> QDSTSDLIPAPPLSKVPLQQNFQDNQFHGKWYVVGLAGNEVLREDKDPMKMWATIYELEEDKSYNVTIVMPLAEKCEYLFQTFVPGSQPGEFTL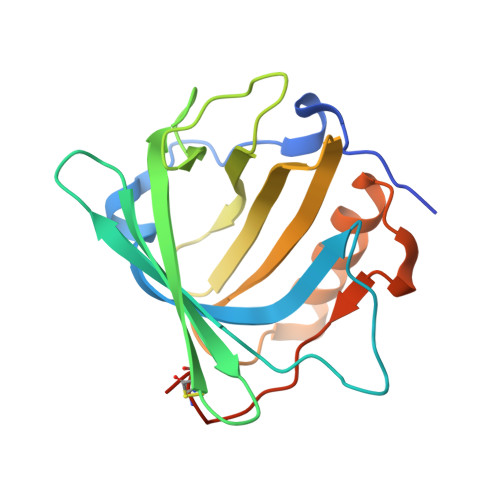GGIKSGPGRTSGLVRVVSTNYNQHAMVFFKVVWQNREVFWVTLYGRTKELTSELKENFIRFSKSLGLPENHIVFPVPIDQCIDGSAWSHPQFEK>[2x]AYVSDVYCEVCEFLVKEVTKLIDNNKTEKEILDAFDKMCSKLPKSLSEEC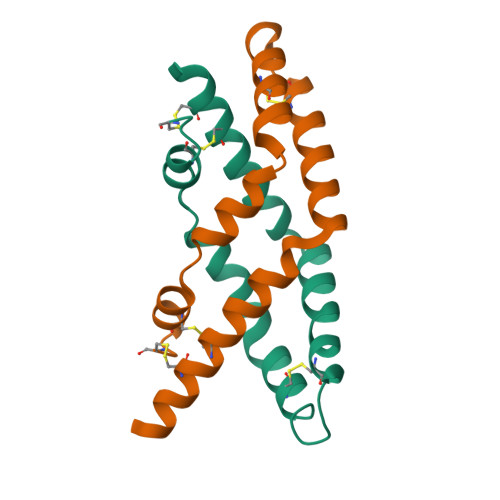QEVVDTYGSSILSILLEEVSPELVCSMLHLCSGTRHHHHHH> MKLSKQKASLLTAVLLLLSLSITTITVDAARVRTYPNVSHANTHYKNTVSSKLLPFTANYQLQLGELDNLNRATFSHIQLQDRHETKDVRTKINYDPVGWHNYQFPYGDGSKSSWVMNRGHLVGYQFCGLNDEPRNLVAMTAWLNTGAYSGANDSNPEGMLYYENRLDSWLALHPDFWLDYKVTPIYSGNEVVPRQIELQYVGIDSSGELLTIRLNSNKES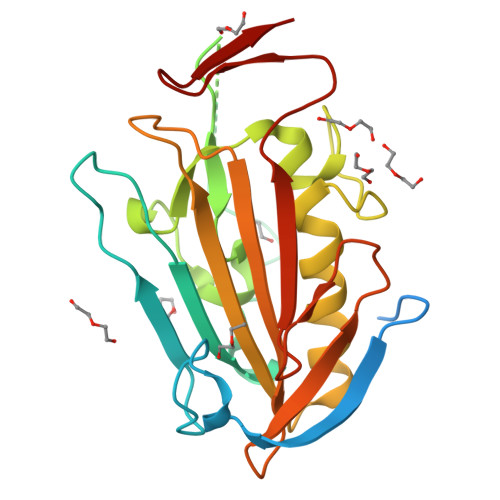IDENGVTTVILENSAPNINLDYLNGTATPKN> NVEEETKYIELMIVNDHLMFKKHRLSVVHTNTYAKSVVNMADLIYK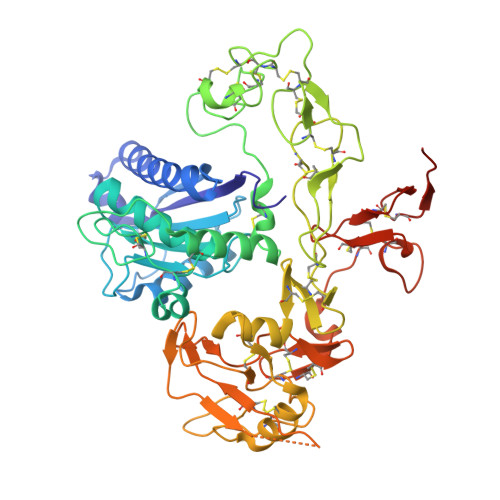DQLKTRIVLVAMETWATDNKFAISENPLITLREFMKYRRDFIKEKSDAVHLFSGSQFESSRSGAAYIGGICSLLKGGGVNEFGKTDLMAVTLAQSLAHNIGIISDKRKLASGECKCEDTWSGCIMGDTGYYLPKKFTQCNIEEYHDFLNSGGGACLFNKPSKLLDPPECGNGFIETGEECDCGTPAECVLEGAECCKKCTLTQDSQCSDGLCCKKCKFQPMGTVCREAVNDCDIRETCSGNSSQCAPNIHKMDGYSCDGVQGICFGGRCKTRDRQCKYIWGQKVTASDKYCYEKLNIEGTEKGNCGKDKDTWIQCNKRDVLCGYLLCTNIGNIPRLGELDGEITSTLVVQQGRTLNCSGGHVKLEEDVDLGYVEDGTPCGPQMMCLEHRCLPVASFNFSTCLSSKEGTICSGNGVCSNELKCVCNRHWIGSDCNTYFPHNDDAKTGITLSG>[2x]LPSSFRWSSSGPLIGPKSDSRRIQGIKDPSVVYHDGRWHVFASTAKTEGYNLVYISFTDWAQAGSASFYYLDQAPLGTGYRAAPQVFYFAPQRLWYLVYQNGNAAYSTNPDINNPAGWTAPRTFYSGMPAIIRNNIGNGHWVDMWVICDSSLCHLFSSDDNGHLYRSQTSLSNFPNGFNEPVIAMQDSNKNRLFEAANVYRIDGSNEYLLLHEAIGSDGRRWFRSWTSTSIAGPWRALADQ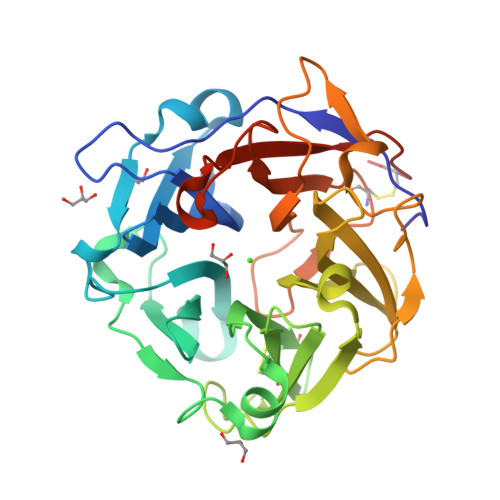ESNPFARANNVAFTGNAWTRDISHGELIRSGNDQTLPISPCNLRYLYQGLDPNSGGDYNSLPWKLGLLTQTNSACAAALEHHHHHH> MVIATDDLEVACPKCERAGEIEGTPCPACSGKGVILTAQGYTLL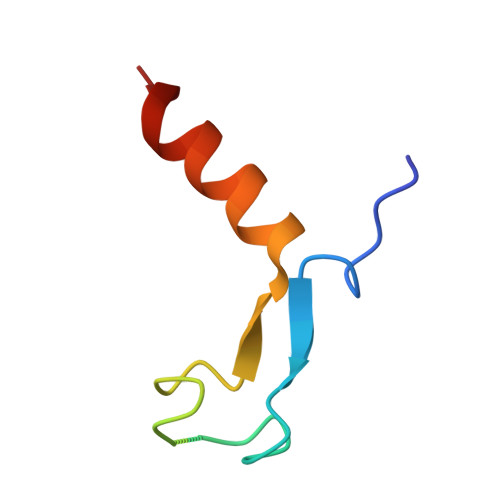DFIQKHLNK>QDSTSDLIPAPPLSKVPLQQNFQDNQFHGKWYVVGMAGNGDLREDKDPYKMRATIYELKEDKSYNVTWVWFLPKKCKYFINTFVPGSQPGEFTLGLIKSYPGQTSLLVRVVSTNYNQHAMVFFKTVIQNRERFYITLYGRTKELTSELKENFIRFSKSLGLP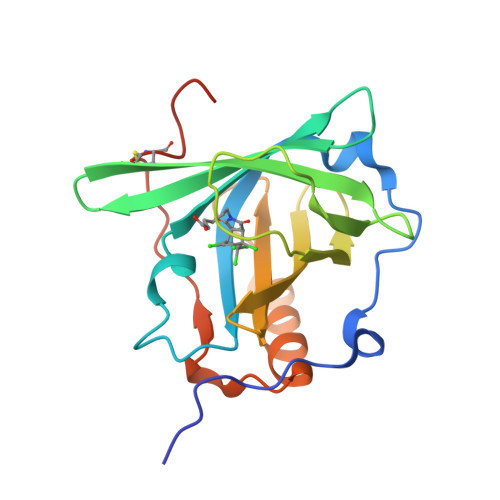ENHIVFPVPIDQCIDGSAWSHPQFEK[3x]>IMEIKKFIETIKGTKLFTAYNTNVDAIKYLKDEDVQKLVDEFNHKDIIERMEEYPRIIEEPLDFVARLVHSIKTGKPAEVPIKDDKKLHEWFDRIKYDEERMGGQAGIVSNLMATLQIDKIIVYTPFLSKKQAEMFVDYDNLLYPLVENGNLVLKKVREAYRDDPIKINRIFEFKKGLKFKLNGEEITAKQSTRFIVASRPEALRIEIKDDVRKFLPKIGEAVDCAFLSGYQAIKEEYRDGKTAKYYFERAEEDIKLLKKNKNIKTHLEFASISNIEIRKMVVDYILSNVESVGMDETEIANVLHILGYDELSNNILKDSFIEDVIEGAKILLDKFKNLEVVQVHTIYYILFVCRADNPLSKEELEECLEFSTILASTKAKLGNIRAIDDLHEGLKIPHNKYGDLLKEIAEKFNDNNY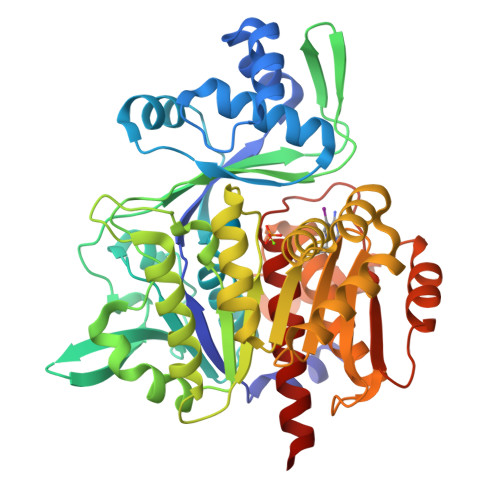KIALSPSRYVEKPKSTVGLGDTISSGAFVYYVSLLNKKRM[3x]>IVGGTNASLGEWPWQVSLQVKLVSQTHLCGGSIIGRQWVLTAAHCFDGIPYPDVWRIYGGILSLSEITKETPSSRIKELIIHQEYKVSEGNYDIALIKLQTPLNYTEFQKPI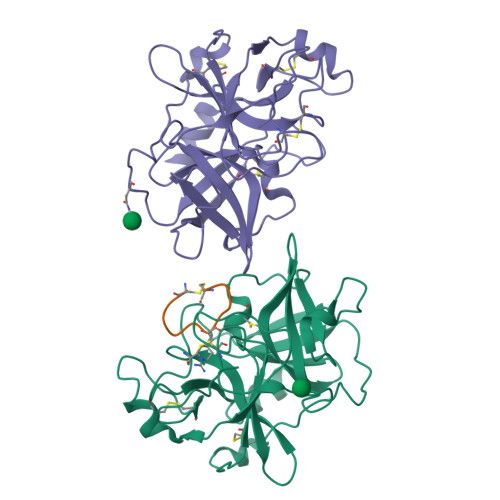SLPSKADTNTIYTNCWVTGWGYTKEQGETQNILQKATIPLVPNEECQKKYRDYVINKQMICAGYKEGGTDACKGDSGGPLVCKHSGRWQLVGITSWGEGCARKDQPGVYTKVSEYMDWILEKTQSSDVRALETSSA[2x];> CPAYSAYLDC>MSGMSPYKKAI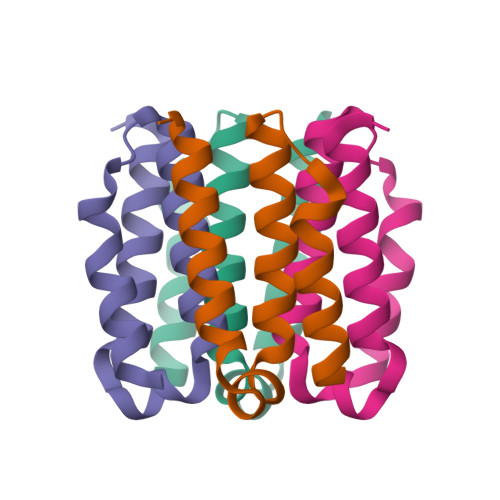EITKRLLELLLSNPELAKKNLGGIATLISLLALISALDGTLDEKDIEPYIKKLEESLGS[2x]3-[(2R)-2-[(benzylsulfonyl)amino]-2-(dihydroxyboranyl)ethyl]benzoic acid | C16 H18 B N 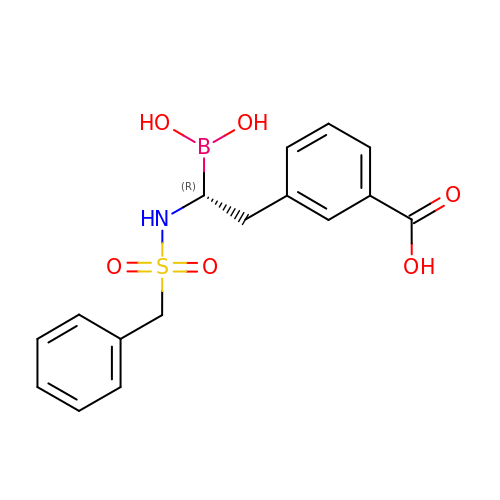O6 S | LCKOZWBVAVBOPR-HNNXBMFYSA-N>[2x]QDGEALFKSKPCAACHSIDAKMVGPALKEVAAKYAGQEGAADLLAGHIKNGTQGNW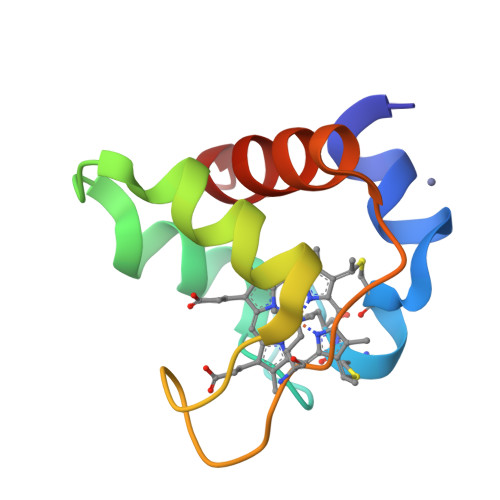GPIPMPPNPVTEEEAKTLAEWVLSLK>[2x]SLDKLHVTSTRPQYVRIKNWGSGEILHDTLHHKATSDFTCKSKSCLGSIMNPKSLTRGPRDKPTPLEELLPHAIEFINQYYGSFKEAKIEEHLA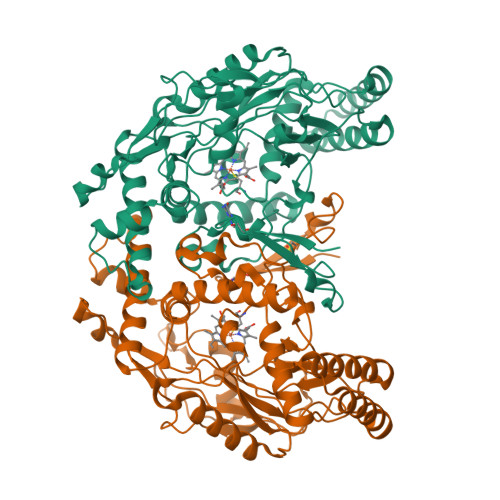RLEAVTKEIETTGTYQLTLDELIFATKMAWRNAPRCIGRIQWSNLQVFDARNCSTAQEMFQHICRHILYATNNGNIRSAITVFPQRSDGKHDFRLWNSQLIRYAGYQMPDGTIRGDAATLEFTQLCIDLGWKPRYGRFDVLPLVLQADGQDPEVFEIPPDLVLEVTMEHPKYEWFQELGLKWYALPAVANMLLEVGGLEFPACPFNGWYMGTEIGVRDFCDTQRYNILEEVGRRMGLETHTLASLWKDRAVTEINVAVLHSFQKQNVTIMDHHTASESFMKHMQNEYRARGGCPADWIWLVPPVSGSITPVFHQEMLNYVLSPFYYYQIEPWKTHIWQNEHHHHHH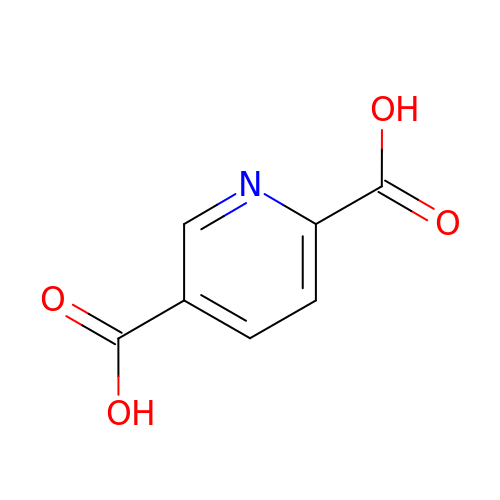pyridine-2,5-dicarboxylic acid | C7 H5 N O4 | LVPMIMZXDYBCDF-UHFFFAOYSA-N>[2x]AAGESMAQRMVWVDLEMTGLDIEKDQIIEMACLITDSDLNILAEGPNLI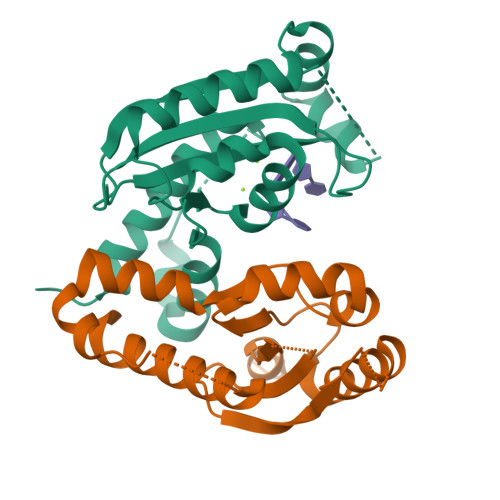IKQPDELLDSMSDWCKEHHGKSGLTKAVKESTITLQQAEYEFLSFVRQQTPPGLCPLAGNSVHEDKKFLDKYMPQFMKHLHYRIIDVSTVKELCRRWYPEEYEFAPKKAASHRALDDISESIKELQFYRNNIFKKK>[2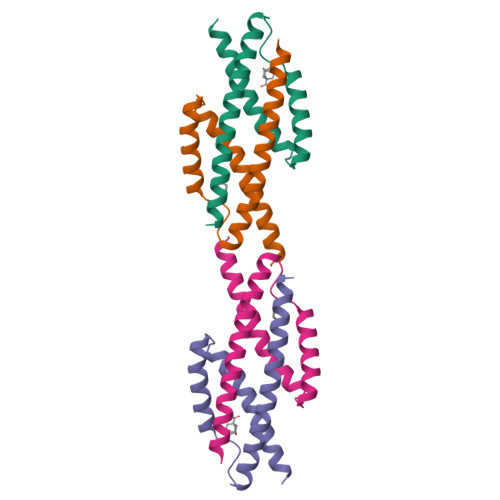x]MTSENPLLALREKISALDEKLLALLAERRELAVEVGKAKLLSHRPVRDIDRERDLLERLITLGKAHHLDAHYITRLFQLIIEDSVLTQQALLQQHLNKINPHSARIAFL>QQDPDPSQLHRSSLVKNLQNIYFLYEGDPVTHENVKSVDQLLSHDLIYNVSGPNYDKLKTELKNQEMATLFKDKNVDIYGVEYYHLCYLCENAERSACIYGGVTNHEGNHLEIP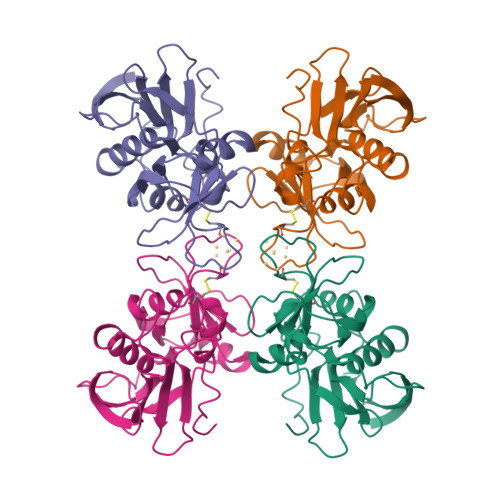KKIVVKVSIDGIQSLSFDIETNKKMVTAQELDYKVRKYTIDNKQLYTNGPSKYETGYIKFIPKNKESFWFDFFPEPEFTQSKYLMIYKDNETLDNKTSQIEVYLTTK[8x]methyl (R)-(2-carbamoyl-5-chloro-1H-indol-3-yl)[3-(2-cyanoethyl)-5-methylphenyl]phosphinate | C20 H19 Cl N3 O3 P | 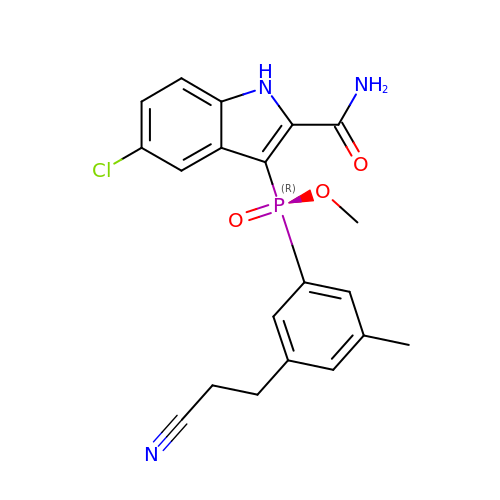KJQCBIWCQKNBKR-MUUNZHRXSA-N> MPQPLVWTQLKQTGTTQPTARSGHTIITVGKTHIMFGGLDNDKNNYKDGKIAPNNQVFTLKLTQNNCEWRQIACQGDVPLPRCYHASCAISADKMLVFGGSYTSNLRFNDTYILKTTSYQWSKPANQISGGEPKNAESKIGAPQPRYGHSATFFEGKVYIFGGHGGINYQRLAFNDLYVLETENFEWTRLEPKGNPPDPRGGHSAAMMANKPQLMIFGGWSFTSQYSNIMIYDIEKDEWVDPEIAHEIPKWNLSGIMAPSIPSWKYFIFGGSVGSFEEGGNRTNSRFVDDSFVLDIDTLSWSSINLEADETSKAVCKPRPRESASIFYDSGESRAIVFGGWANNWLNDLWALNVSTITGPPYAIFSIKPALGPLTGKTKVLIEGDGFKDTQNISVKFSGGKLEKEVNGTFVNEKEISCETPTFDYPRSVEVTVCMNKGDYTITKSAFTYYLNTKADKTIAYGPGLLTENLIGVQTTIVIQARNKNDQNRESGSDEFVVTIRNPAKIKKEEEVKEGDKANTKNTIKEDEEEEGEDEEENKKKKEAEKAAAEKAAAEKAAEEEQGEAVDPSLVPFNIVDNDDGSYFIQFTSEEEAVLEIDIKFKDENNELHSIRGNPFRCGFVKGSKPNNNDLTGSAVMNYISKQLKDIQEFIENTKENIEIRNKNIRENVSELINVMINLEKVRVKNDDDVLTLDTVEEMLNFLKKKDFGKDSDIKKCKKLQEEWKNLAKMAQAVKKDIQNPVKTESDKTKENIKKFEEITLKEYANSLKKESFFIYKTGVSESFKRIGEVKQKVDEFEVQLNQYEDFARMFEFPDAVIGSKKLMEQIRTDVSSVEKLWVRIEISEKTMDEYKKMKWGSINSMDMEDEIKKLRKALTDLRGIDKRSNAFIGITEELKKWATFLPLLGELKDPSMNSEDGRHWKKLKDLVKKEFDVSQELMLEIIWDLKLFDYKDGIEEITDQAKQELKMEKALKKIIDFWRDIEFELVQHKNTDIHTLKMSEENFETLEDHQLQINNMLLSKYVAYFEKEVEKWKYDLGSVYDVVQLLLEVQKTWSFLENLFIQSEEVKRELPNESAQFVGIDKDMKEIMQKGCDIKNCLKFCTIEGMLKRLENIQAQLKVCEKALNEFLDSKRRAFPRFYFVSVNDLLDILSNGNSPAKINRHMSKIFQAIDNLQLKEDSSGGRPTALKMISCVGTEEVDFSSPRLLQGKVESYLKDVIDTMIGTLKSVANSSFKNFQSMTRKEWLKSDPSQITLLVNNIIWSKAVEDCFLKLQSGDINAMKLFLDESIKQLTELIGMVQGDLSKPLRQKIMCLITIDTHSRDVVHRLINEHVRKAEEFQWQSQLKFYWVDNDAKIKIADARFVYNYEYLGNGPRLVITPLTDRIYVTATQALHLKMGCAPAGPAGTGKTETTKDLANALAKACYVFNCSSEMNYESMGNIYKGLASSGCWGCFDEFNRLLPEVLSVCSVQFKAVTDAIKQNVERFIIEGDEISLDPTCGVFITMNPGYLGRAELPEGLKALFRPITVVVPDLELICENMLMAEGFIEAKILAKKFVTLYMLCRDLLSKQLHYDWGLRAIKSVLVVAGGFKRSEPEIAEQALLMRALRDFNIPKIAFQDLYVFHGLLGDLFPGINIKPKKDLDFEKIITDVCIENKLDPDPEFVLKVVQLSELLAIRHCVFVMGPPGAGKSTTWKILAKAQDKTNKKTTLIDIDPKVVSTKDFYGYNLPSKEWKDGLFSKMLRSLAEQPDTNPKWICLDGDLDANWIESMNSVMDDNKILTLANNERIPLKPHMRALFEIRDLRFATPATVSRAGILYISDEVGYQWRSYVKSWIKQEFSQDQEMSKNLDTLFGKYVPDTLDHIKKHCRFLVPVSPISQVISICKSLQTLLKGDVKNLEYLFVYALIWAIGGALAEKDSIDYRKDFSTWWKGAWKTAVKFPSKGTIFDYYVDQSGDSSKFVEWSKRLENKEFDPQVETMGNITVNTIETLATTEFIKSYLMVKHPSLLIGNSGCGKTQLAKGILKEIVQAKPENYAYQLIN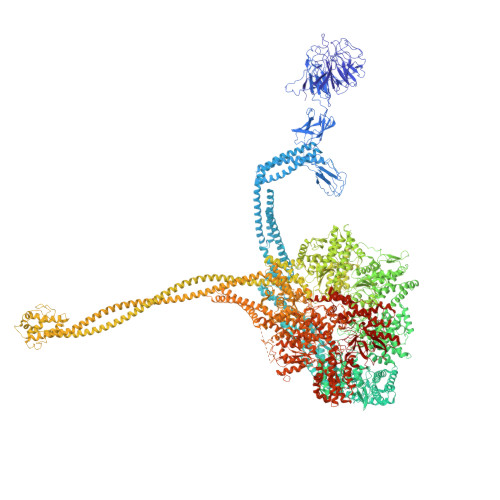FNYYTDSTYLQGQIEQTLEKKAGRQYGPPGKVQLIYFIDDLNMPQLDAYDTQTAIALLRQLADYGHFYDVSKLALKDIINTQVLAAMNPSAGSFFVNPRYQRHFWTISIPFPDNESLSLIYITFLNGHLKRFKSTIQEYSNIIVRASLMLHQAVTQNFRKTAINFHYEFNLRHMSNVFQGLLLSDPNKFTEPDKLIKLWIHECERTYGDRLVSTDNLKTYKENIFDIVKKSFSKFNFSRYFGNNPENLIYCNFIAGINSDRFYDQMPNNEMEKHISEALKEYNDNNAFMGLVLFEDAMKHVCRICRIVLPSSGHALLVGVGGSGKQSLSKLASFIMGYTTFSITISATYSMVDLRNDLQQLYFKCGPKEEGILFLFTEGQITNERFLVYINDLLSSGEIAELYTLDEKEAMINQVRAKVKGEGKPDTRENCWNWFIDQVKKNLHMAICFSPVGDMRRRARQFPALVNCTVIDWFQPWPYEALFNVAKSFLEPVDLGDDKVREAVVKFMPFSFTLVNDLGLKLLEQERRYAYTTPKSFLELISLFTNMLAQKRESLERNKERYETGLVKLKETAEQVAIIEVEVKEKQVEAEAKKKEADAFAEVVGREKDKVEKENSKATIEADKCGLIKQNVEAQKSSTQQDLDAAQPLVEQAKSALNSISKKDFQQAKSFASPPAGVPEVFAATIYLLAGYFNEAIEIDKNKKPKDVSWKSSLKLMKSPEEFMEKLLNFKDVVDANQVPAANVNIVKNQYLNMPSFTPEQMASKSAAAKGICSWVVNIVKYYDVIQDVEPKRKALKEATEQLEEATVKLNEVEEVVRKLNEELNKLKAENDKAIAERNAAISEAERCARRLNLAQRLVTALSSENERWGKSIIQLEDQLKLMVGDVLVASSFVSYSGPFNKKFRNIMINQNFMKFMKEHTIPMSPDPNPIKILTDESTIALWNKQKLPSDSVSIENGTILTNSARYPLMIDPQLQGITWIREKEKANNLKILRLGSKNINRDLELSIENGYSAIIENMNERIDAILMPIIARSFIKRGKNKIIKFAGKDLILHPNFKLFLHTKLSNPHYPPEIQAEAALINFTVTEAGLGDQLLSLVVARERPDLAKMKIELITQQNDFKIKLKDLEDELLYKLANAKGDILDDIELIENLEYSKKLSVEIAEKVAAAKITEAKINETSENYRPAASRGALFYFLLSDLSKVHSFYKYSLESFIVVINRAIDAISENKIYGKTTMVPYGDETYASNQHEKEEEEEEEEHQQAQQQQNQEEQQEQKDEENKGPVEEEQPEGENKGPVEEEGAEGQNEGPVEEENAENQEGEGEEEGEKQQKAKDSDEPMSPRSLKKRVDELIESLTYTAYQTTRRGLFESHKLIVAAMLCLRVLLRSEELNSDEVDHLIIGKVDVNPTPMPDALKSFLNDNIWAACKALETIHQFQGFCQSLETDVLQWKKWYSEEKAETADLPKAFKELSKFHRLLLLRALRPDRLPSALSQFVHDKMGERYIEQPPFNIFETFQETSKTVPIFFVLFPGVDPTPDVERVAATFDVSANNGRFINISMGQGQEDRAKKALFDCAQKGHWIMLQNVHLMQSWLYGLNGLEGFLESVFASPKTHPNFRVFISSEPPNVLLPLMQIIPESILQGSLKIANEAPQYLKANLRRAYNKFDQEFLDKCDKKPTEFKSCLFALCFFHSLMLGRKKFGTQGWSRVYNFNDGDLTICADVLYNYLSKYDQVPWDDLRYIFGEIMYGGHITDDWDRRTNRTYLKVLIRSELLQQNFNLAPQFKSPDPSKFDYEAYRKYIEEKLPIESPQMFGMHPNAEIGYLTQTCDQVFNTILEVQGGSSGGGASKKDDGVMVTLTDFKTRCPHDFNMLLIEEKVKEKTPYIVVCLQECERMNGLLKEIKTSLEDLRLGLTGALNMTDAMESLQQSLSFNKVPDTWEKKAYFSKKPLSSWFADLIERNIQLQEWCKELVTPTSLCISYLFNPMSYLTAIMQFTARAQGLPLDGITIQTNVTAMKGPEDVVNPAENGAYIHGLFLEGAAWEIGGQGQDGYLIEQKPKELHPKMPVINAVAVPLDKKKKNGQYDCPTYVTSARGQTFVFTANLNMESDDSDPNKWILSGTCMLMSDD> MPKFLDALAGFAVTLGSMFKKPITEGYPEKPGPVAPRYHGRHQLNRYPDG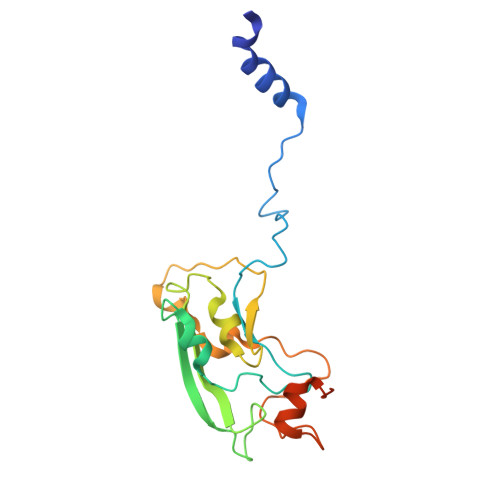LEKCIGCELCAWACPADAIYVEGADNTADERYSPGERYGRVYQINYLRCIGCGLCIEACPTRALTMTTEYEMADDNRADLIWGKDKLLAPLQEGMQAPPHDMAPGKTDDDYYLGNVTPITPVPSGTEDAR>[3x]MKNNLPIIALDFASAEETLAFLAPFQQEPLFVKVGMELFYQ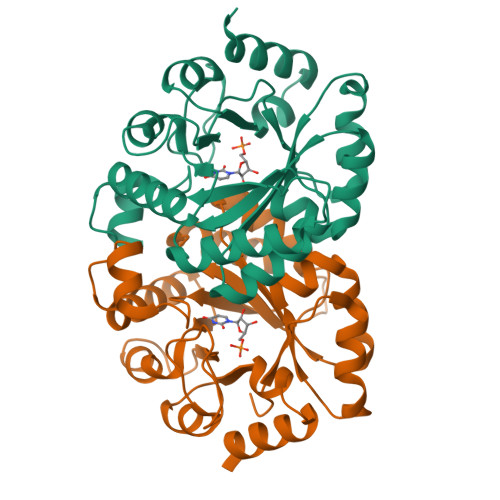EGPSIVKQLKERNCELFLDLKLHDIPTTVNKAMKRLASLGVDLVNVHAAGGKKMMQAALEGLEEGTPAGKKRPSLIAVTQLTSTSEQIMKDELLIEKSLIDTVVHYSKQAEESGLDGVVCSVHEAKAIYQAVSPSFLTVTPGIRMSEDAANDQVRVATPAIAREKGSSAIVVGRSITKAEDPVKAYKAVRLEWEGIKS The NpnN, Ap4A, Ap5A and Gp4G levels within cells are primarily maintained by Nudix hydrolase superfamily member Ap4A hydrolase (Ap4AH from hereon). Based on sequence analysis the P. falciparum Ap4AH (PfAp4AH, EC 3.6.1.17) was predicted to be an animal-archeal type which cleaves polyphosphate chain at the fourth phosphate from the tightly bound adenosine resulting in asymmetrical cleavage of Ap4A. PfAp4AH can asymmetrically hydrolase Ap4A and Ap5A molecules produced by PfKRS (and probably by other Pf aaRSs) to ATP + AMP and ATP + ADP, respectively. PfAp4AH folds into a conventional Nudix domain, with four β-strands (β1, β2, β4 and β5) sandwiched inside two anti-parallel helices (α1 and α3).

We also provide two crystal structures of PfAp4AH - in apo and sulphate-bound forms at atomic resolution. There are four molecules in asymmetric unit for PfAp4AH-apo and designated as A, B, C and D. The atomic resolution structure of PfAp4AH-SO4 has three SO4 ions and a PEG molecule which arise from crystallization buffer. Of the three SO4 ions bound in PfAp4AH-SO4, one engages the P1 site (located between loops L2 and L5). We were able to directly compare the active site residues involved in engaging sulphates (or P1 by analogy). Active site-bound SO4 is coordinated by analogous residues (Pf/Hu) His43/His32, Lys48/Lys42 and Tyr87/Tyr82, but unlike PfLys94 analogous HsLys89 does not engage sulphate. Global structural differences between apo- and SO4- bound PfAp4AH were apparent upon superimposition. Three major variable regions arising from SO4 binding and different space group packing of PfAp4AH were identified in loop regions L2, L3 and L5 and analyzed further. In case of PfAp4AH-SO4, His51 forms a hydrogen bond with one of the water molecule in a nearby water network linked to Ser56. In particular, side chain flip in Tyr87 and His43 suggests substrate-induced conformational adjustment similar to the human counterpart.

> MKINIIKAFGILLCRLKKYNPVTTGDINKFEFLFLKASYADKHWTPPKGLHENNESGLETAVRETLEETGINKDKYKLLNYQKTLKYNVKDKPKETTYYLAMLLNNEENVILSDEHTDYKWIGSHESDTYNLPESLADLLKEAEEFLNKEQL Microbial rhodopsins (MRs) are transmembrane light-sensitive proteins, found in Archaea, Bacteria, Eukaryota, and also viruses. MRs are composed of seven transmembrane α-helices (A–G) with the cofactor retinal covalently bound to the lysine residue of helix G via the Schiff base (RSB). Despite this paradigm, the first light-driven Na+ pump KR2 was identified in Krokinobacter eikastus in 20132. KR2 contains a characteristic for all known Na+-pumping rhodopsins (NaRs) set of N112, D116, Q123 residues in the helix C (NDQ motif).

To verify that flash-cooling does not affect the conformation of the O-state, we solved X-ray structures of the illuminated KR2 at room temperature (RT) during continuous 532-nm laser illumination using both single-crystal and serial millisecond crystallography. These approaches allow to detect the dominant conformational changes of the photocycle. Structure refinement identified nearly 1/1 ratio of the ground/O-states populations in crystals in both cases. The structures of the O-state at RT are identical to each other and also to that at 100 K, which indicates that cryo-cooling does not affect the O-state of KR2.

>[5x]QELGNANFENFIGATEGFSEIAYQFTSHILTLGYAVMLAGLLYFILTIKNVDKKFQMSNILSAVVMVSAFLLLYAQAQNWTSSFTFNEEVGRYFLDPSGDLFNNGYRYLNWLIDVPMLLFQILFVVSLTTSKFSSVRNQFWFSGAMMIITGYIGQFYEVSNLTAFLVWGAISSAFFFHILWVMKKVINEGKEGISPAGQKILSNIWILFLISWTLYPGAYLMPYLTGVDGFLYSEDGVMARQLVYTIADVSSKVIYGVLLGNLAITLSKNKEL> GASEPMRPGVIRFGLTPVFLSNDLEVLDELQAYLTQAVGQEVQLITQRTYQEVTALLVSGNLEAAWICGYPFMKFRDELDLVATPLWRGKPVYQSYLIVGRDRDIAGFEDCQGDIHAFSDPDSNSGYLVTKTYLAERGVSEEGFFRKSFFTYGHRNVIRAVASGLADSGSVDGYVWEVMKTTEPELVAKTRVLVKSGWHGFPPVAAAAGQRKSQAVARIRSALLDMNQEVLGRSVLTRLQLDGFVETTAESYDSIAANMERVRRLG

The regulatory cluster consists of three genes, aioX, aioS and aioR, which encode a periplasmic-binding protein (PBP), a sensor histidine kinase and a response regulator, respectively. Arsenite-bound AioX is thought to act as a ligand for AioS, the sensor histidine kinase that upon auto-phosphorylation, phosphorylates AioR, the response regulator, which binds to a conserved sequence upstream of a RpoN promoter. AioX exhibits a typical bilobed structure of the PBP type II class. In this class of proteins, the ligand-binding pocket is located in the space between the two domains.

While the majority of both structures overlay very well, there is a significant difference in the rotamer conformation of Tyr88. The change in the side chain conformation is further associated with the backbone shift for residues 83–88 and a significant conformational change in the loop region comprising residues 53–61, demarked by the black circle in Fig. 5A. It should be noted that while surface residues 59–61 in the arsenite-bound structure are near the neighbouring molecule in the asymmetric unit, they are too distant to be directly involved in the interactions, while in the apo-AioX Asp61 interacts with the side chain of Arg281 from the crystallographic symmetry related molecule. These small differences in molecular packing support the idea that 53–61 loop conformation change might result in the generation of a new protein interaction surface. The fact that the arsenite-bound and apo-AioX crystals displayed differences in molecular packing (forming weak local and crystallographic symmetry related dimers, respectively) supports the idea that loop conformation change might result in the generation of a new protein interaction surface.> ALAEVQARHQELLKLEKSMAELTQLFNDMEELVIEQQENVD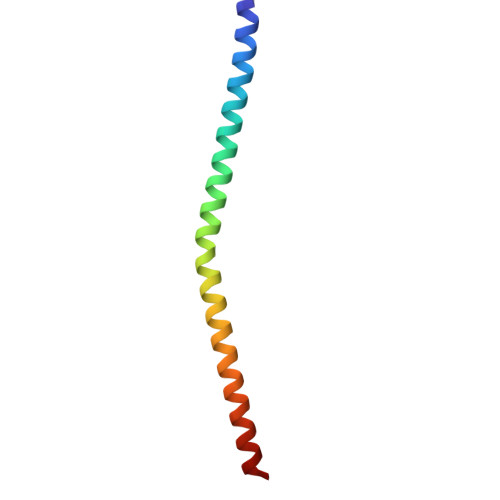VIDKNVEDAQLDVEQGVGHTDKAVKSAR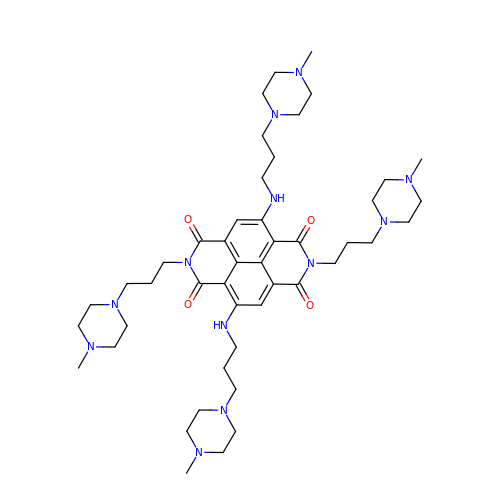2,7-bis[3-(4-methylpiperazin-1-yl)propyl]-4,9-bis{[3-(4-methylpiperazin-1-yl)propyl]amino}benzo[lmn][3,8]phenanthroline-1,3,6,8(2H,7H)-tetrone | C46 H72 N12 O4 | KISMKSDSZPCOMD-UHFFFAOYSA-N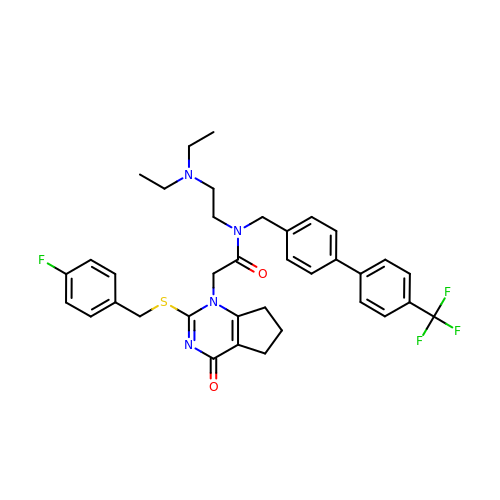N-[2-(diethylamino)ethyl]-2-{2-[(4-fluorobenzyl)sulfanyl]-4-oxo-4,5,6,7-tetrahydro-1H-cyclopenta[d]pyrimidin-1-yl}-N-{[4'-(trifluoromethyl)biphenyl-4-yl]methyl}acetamide | C36 H38 F4 N4 O2 S | WDPFJWLDPVQCAJ-UHFFFAOYSA-N>MGSSHHHHHHSQDPIRRGDVYLADLSPVQGSEQGGVRPVVIIQNDTGNKYSPTVIVAAITGRINKAKIPTHVEIEKKKYKLDKDSVILLEQIRTLDKKRLKEKLTYLSDDKMKEVDNALMISLGLNAVAHQKN[2x]

TA modules are small operons encoding two proteins: a ‘toxin’ that interferes with basic cellular metabolism, usually translation or transcription, and an ‘antitoxin’ that neutralizes the toxin and protects the cell from its potentially destructive activity (for reviews see 1–4). The toxin MazF is activated under a number of stressful conditions via proteolytic degradation of its neutralizing antitoxin MazE by the ClpPA or Lon proteases, (18,30,35) and was proposed to be under control of quorum sensing. In this paper, we present a method to obtain large quantities of active SaMazF and provide the structure of this protein as determined by nuclear magnetic resonance (NMR) and X-ray crystallography. The SaMazF dimer is formed by pairing strand S6 from two monomers to form a dimer-wide 10-strand anti-parallel β-sheet.

Three different crystal forms of SaMazF are available, which lead to the structures of 14 crystallographically independent SaMazF monomers forming 7 independent dimers. In particular, among the two loops that show higher RMSD values in the X-ray ensemble, loop S3-S4 (Gly48-Lys54) is involved in lattice contacts in all structures. It is unlikely, however, that crystal lattice interactions have a major influence on the conformation of this rather extended loop given that all conformations observed seem to belong to a single family, with only two individual conformations (form I chain D and form II chain A) deviating somewhat from the canonical conformation. Loop S4-S5 (Ile61-Lys70) is involved in lattice contacts in most but not all SaMazF monomers. Four classes of conformations are observed. The most common conformation is observed in ten chains, two cases of which do not involve lattice contacts. In the remaining four chains, this conformation is prohibited as it would lead to steric clashes with a neighboring monomer. Of these remaining chains, form II chains A and B adopt the same conformation while form III chains D and E each adopt a unique conformation. Loops S4-S5 of the latter four chains are all involved in lattice contacts. Thus, it seems like loop S4-S5 will adopt a default conformation when the crystal environment allows for it, but will adapt its conformation otherwise.> GMSQPKKRKLESGGGGEGGEGTEEEDGAEREAALERPRRTKRERDQLYYECYSDVSVHEEMIADRVRTDAYRLGILRNWAALRGKTVLDVGAGTGILSIFCAQAGARRVYAVEASAIWQQAREVVRFNGLEDRVHVLPGPVETVELPEQVDAIVSEWMGYGLLHESMLSSVLHARTKWLKEGGLLLPASAELFIVPISDQMLEWRLGFWSQVKQHYGVDMSCLEGFATRCLMGHSEIVVQGLSGEDVLARPQRFAQLELSRAGLEQELEAGVGGRFRCSCYGSAPMHGFAIWFQVTFPGGESEKPLVLSTS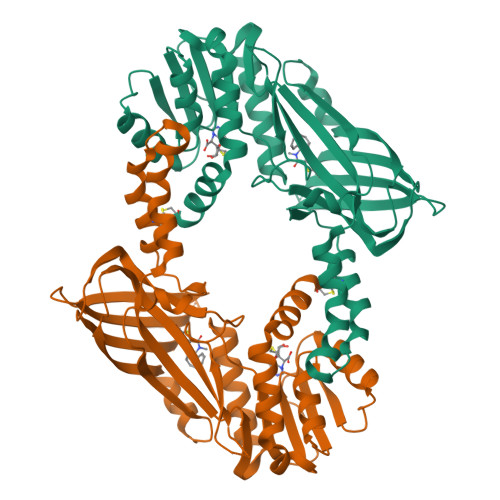PFHPATHWKQALLYLNEPVQVEQDTDVSGEITLLPSRDNPRRLRVLLRYKVGDQEEKTKDFAMED(2R,4S,6S)-4-azanyl-4,6-dimethyl-oxane-2,5,5-triol 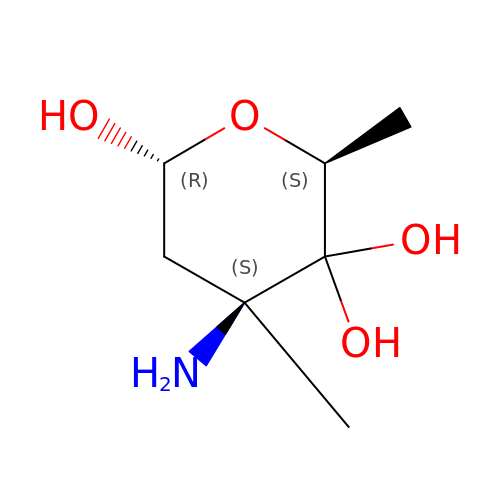| C7 H15 N O4 | ATGUYZRYRGIDLC-JKUQZMGJSA-N> MEHEKDPGWQYLRRTREQVLEDQSKPYDSKKNVWIPDPEEGYLAGEITATKGDQVTIVTARGNEVTLKKELVQEMNPPKFEKTEDMSNLSFLNDASVLHNLRSRYAAMLIYTYSGLFCVVINPYKRLPIYTDSCARMFMGKRKTEMPPHLFAVSDEAYRNMLQDHENQSMLITGESGAGKTENTKKVICYFAAVGASQQEGGAEVDPNKKKVTLEDQIVQTNPVLEAFGNAKTVRNNNSSRFGKFIRIHFNKHGRLASCDIEHYLLEKSRVIRQAPGERCYHIFYQIYSDFRPELKKELLLDLPIKDYWFVAQAELIIDGIDDVEEFQLTDEAFDILNFSAVEKQDCYRLMSAHMHMGNMKFKQRPREEQAEPDGTDEAEKASNMYGIGCEEFLKALTKPRVKVGTEWVSKGQNCEQVNWAVGAMAKGLYSRVFNWLVKKCNLTLDQKGIDRDYFIGVLDIAGFEIFDFNSFEQLWINFVNEKLQQFFNHHMFVLEQEEYAREGIQWVFIDFGLDLQACIELIEKPLGIISMLDEECIVPKATDLTLASKLVDQHLGKHPNFEKPKPPKGKQGEAHFAMRHYAGTVRYNCLNWLEKNKDPLNDTVVSAMKQSKGNDLLVEIWQDYTTQEEAAAKAKEGGGGGKKKGKSGSFMTVSMLYRESLNNLMTMLNKTHPHFIRCIIPNEKKQSGMIDAALVLNQLTCNGVLEGIRICRKGFPNRTLHPDFVQRYAILAAKEAKSDDDKKKCAEAIMSKLVNDGSLSEEMFRIGLTKVFFKAGVLAHLEDIRDEKL

Subsequent studies in C. elegans, Xenopus, Zebrafish, and Drosophila confirmed the role of UNC-45 as a myosin-specific chaperone, promoting the folding of the myosin ATPase domain as well as coordinating the assembly of thick filaments during muscle development. To better understand its myosin folding function, we established an orthogonal protein folding assay in insect cells, characterizing the interplay of the C. elegans muscle myosin MHC-B with its cognate chaperone UNC-45. Structural data of various functional mutants clarify the role of the distinct UNC-45 domains in this process providing important mechanistic insight into its myosin folding activity.

To this end, we used the motor domain of C. elegans body wall muscle myosin MHC-B as model system and co-expressed it with different C. elegans chaperones in insect cells. Finally, we crystallized MHC-B and determined the structure of the ADP-bound state to a resolution of 1.9 Å. The motor domain adopts the canonical myosin ATPase fold being comprised of the N-terminal, the central (upper and lower 50 kDa region) and a C-terminal domain, with all residues (except loops 198–210 and 633–650) being well-defined by electron density. Indeed, the nucleotide binding site of MHC-B is virtually identical to that of the human beta cardiac myosin, with the sidechains that coordinate ADP present in almost identical position. Upon elevating the actin concentration, we observed a 6-fold increase of its basal ATPase activity, which inclined from 0.043 ATP s−1 in the absence of actin to a Vmax of 0.257 ATP s−1. Using similar stopped-flow experiments, we carried out a broad kinetic characterization of the MHC-B myosin motor, determining the rate constants of ATP and ADP binding to myosin and the actin:myosin complex, respectively. In conclusion, the kinetic data demonstrate that the MHC-B variant produced in insect cells is a fully functional myosin motor, which exhibits similar kinetic properties to other muscle myosins. In contrast to the human protein, which has to be produced in a special mouse cell line requiring time- and resource-demanding procedures, the biochemical and structural analysis of MHC-B was performed with a recombinant protein that can be produced in large amounts in insect cells (15 mg myosin per liter cell culture) and is easily accessible to genetic manipulations. Considering the high yields and the overall similarity to mammalian muscle myosins, including the human beta-cardiac variant, the recombinant MHC-B should represent a valuable model system to address the assembly, function and regulation of muscle myosins in basic and in medical research.>MAHHHHHHVDDDDKPGPALYEENALKGKIDDPNSYVPDAVQEAYKNLDSTSTLTEENFGKPYISAKDLKEIMYDHLPGFGTAFHQLVQVICKIGKDNNLLDTIHAEFQASLADGDSPQCALIQITKRVPIFQDVPPPIIHI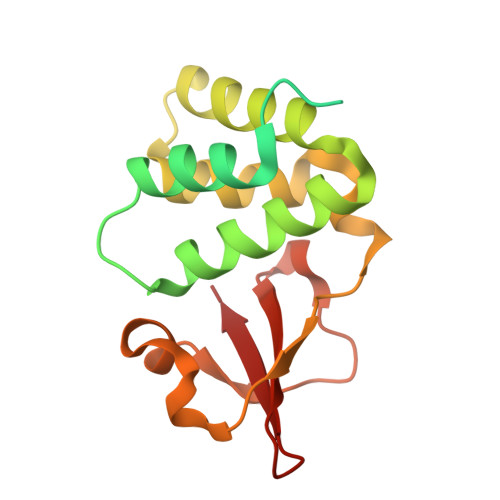RSRGDIPRACQKSLRPAPPSPKIDRGWVCLFKMQDGKTLGLKI[2x]> MASSSTAYYLKDAGFH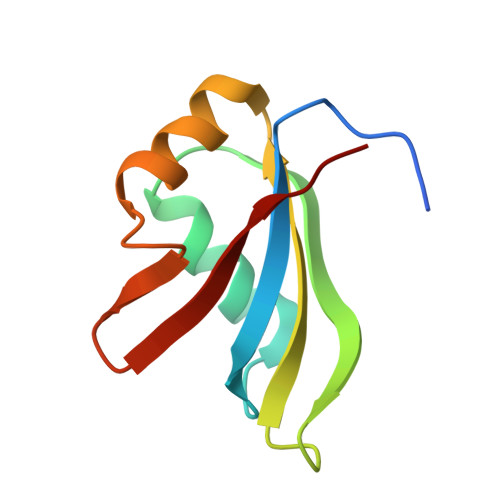IRNIPKAWNDWNLFHVFQNFGKVSYCRVVGQSNDGQVQLGFVNMMSVADADEVRKNLNDGNLIGENFTLKVTDHKN>MDSKHQCVKLNDGHFMPVLGFGTYAPPEVPRSKALEVT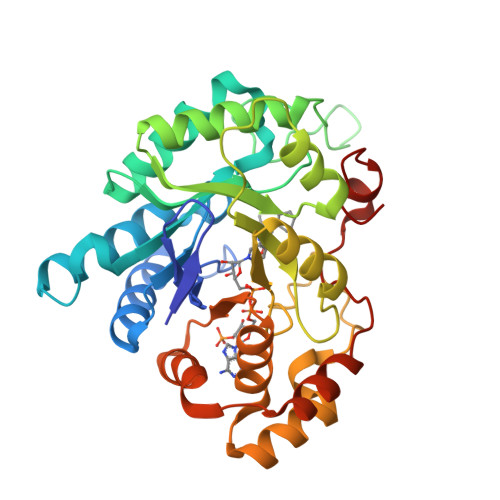KLAIEAGFRHIDSAHLYNNEEQVGLAIRSKIADGSVKREDIFYTSKLWSTFHRPELVRPALENSLKKAQLDYVDLYLIHSPMSLKPGEELSPTDENGKVIFDIVDLCTTWEAMEKCKDAGLAKSIGVSNFNRRQLEMILNKPGLKYKPVCNQVECHPYFNRSKLLDFCKSKDIVLVAYSALGSQRDKRWVDPNSPVLLEDPVLCALAKKHKRTPALIALRYQLQRGVVVLAKSYNEQRIRQNVQVFEFQLTAEDMKAIDGLDRNLHYFNSDSFASHPNYPYSDEY[2x]(phenylmethyl) 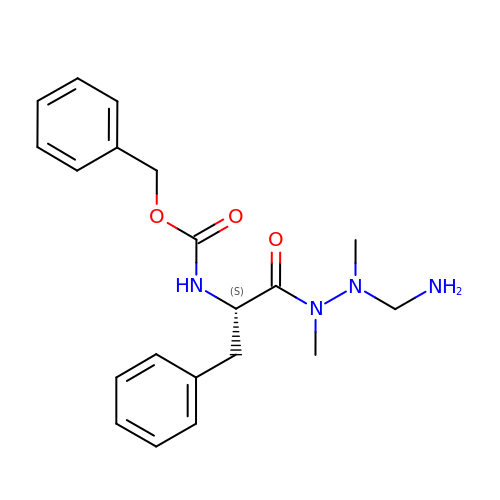~{N}-[(2~{S})-1-[[aminomethyl(methyl)amino]-methyl-amino]-1-oxidanylidene-3-phenyl-propan-2-yl]carbamate | C20 H26 N4 O3 | OUWJIALCFGQZPQ-SFHVURJKSA-N In S. cerevisiae meiosis I, sister kinetochores are fused through the action of the kinetochore-binding monopolin complex, and together bind a single microtubule. The conserved core of the monopolin complex comprises two nucleolar proteins, Csm1 and Lrs4. These proteins form a distinctive V-shaped complex, with two Csm1 homodimers bridged at their coiled-coil N-termini by a pair of Lrs4 subunits, thereby positioning two pairs of Csm1 globular-domain “heads” ~ 10 nm apart at the apices of the V. Each Csm1 globular domain has a conserved hydrophobic cavity implicated in binding the kinetochore protein Dsn1, leading to the proposal that monopolin could bridge Dsn1 molecules from sister kinetochores to physically fuse the kinetochores. A ~ 40-residue region within the disordered N-terminus of the core kinetochore protein, Dsn1, has been identified as the kinetochore receptor for the monopolin subunit Csm1.

Mam1, which is found only in point-centromere fungi, binds Csm1 and Hrr25 independently, through two flexibly linked domains, thereby acting as a molecular tether to recruit Hrr25 to the monopolin complex. We also determined a 3.0 Å-resolution structure of Cg Csm169–181 in complex with the Csm1-binding region of Cg Mam1 (residues 162–216). In the crystal structure of Sc Csm1:Mam1, Mam1 forms an extended interface with Csm1 that includes an α-helix binding to the “side” of Csm1 and a phenylalanine residue (Sc Mam1 F262) inserted into the conserved hydrophobic cavity of Csm1. As these data are difficult to reconcile with our finding that Dsn1 Box 2-3 interacts with the same surfaces on Csm1, we determined a new crystal structure of a Cg Csm169–181:Mam1162–216 complex. This structure closely resembles our earlier structure of the S. cerevisiae complex, but does not include an ordered α-helix or any interaction with the Csm1 hydrophobic cavity. Closer inspection of sequence conservation in Mam1 orthologs reveals very poor conservation beyond the “core” region of Mam1 that interacts with Csm1 in our new structure, suggesting that the additional interactions observed in our earlier structure of the S. cerevisiae complex represented non-specific crystal packing interactions rather than a biologically relevant interface. Thus, our new structural data support the idea that Mam1 and Dsn1 Box 2-3 can bind simultaneously to a Csm1 protomer, rather than competing for Csm1 binding. Interestingly, our structural modelling suggests that Mam1 is positioned close to the solvent-exposed residues on the Dsn1 Box 2 α-helix, suggesting a potential further interaction that could stabilise the ternary complex and explain the role of these residues in Dsn1 Box 2.

>[2x]ETIEIIKDLFEHLCGVRVHRTYEDDTGLWFDTSQGSKNGIMDYKLGFVKSQAENTTEVDTEVIYVPLLKQRTAEELQELQKKLPDYLFETLSFPLRSLNQFYIKMSKSLNKKV;>[2x]NVQKYIPPTILTKRRNMESFNDCKVNTKDIISFKDVNQEYETWLDKHLSLAKDRD> MH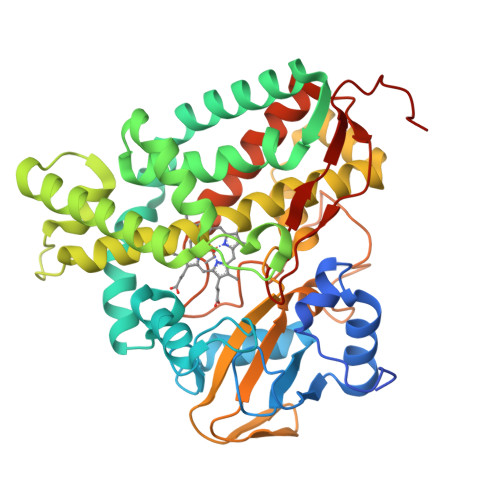HHHHHMPSPNLPMPSPNLPPGFDFTDPAIYAERLPVAEFAELRSAAPIWWNGQDPGKGGGFHDGGFWAITKLNDVKEISRHSDVFSSYENGVIPRFKNDIAREDIEVQRFVMLNMDAPHHTRLRKIISRGFTPRAVGRLHDELQERAQKIAAEAAAAGSGDFVEQVSCELPLQAIAGLLGVPQEDRGKLFHWSNEMTGNEDPEYAHIDPKASSAELIGYAMKMAEEKAKNPADDIVTQLIQADIDGEKLSDDEFGFFVVMLAVAGNETTRNSITQGMMAFAEHPDQWELYKKVRPETAADEIVRWATPVTAFQRTALRDYELSGVQIKKGQRVVMFYRSANFDEEVFQDPFTFNILRNPNPHVGFGGTGAHYCIGANLARMTINLIFNAVADHMPDLKPISAPERLRSGWLNGIKHWQVDYTGRLPVAH> DGLY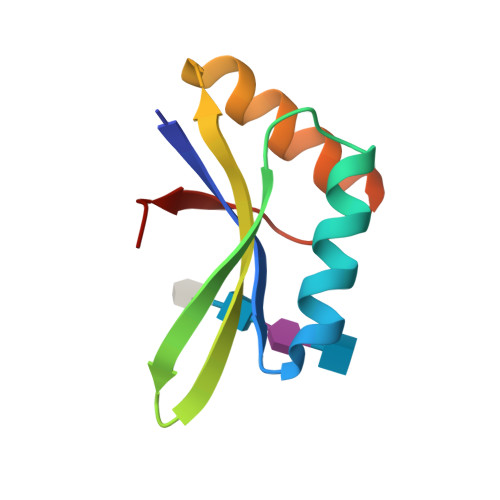LQVGAFANPDAAELLKAKLSGVTAAPVFISSVVRNQQILHRVRLGPIGSADEVSRTQDSIRVANLGQPTLVRPD2-(2-ACETYLAMINO-4-HYDROXY-6,8-DIOXA-BICYCLO[3.2.1]OCT-3-YLOXY)-PROPIONIC ACID | C11 H17 N O7 | 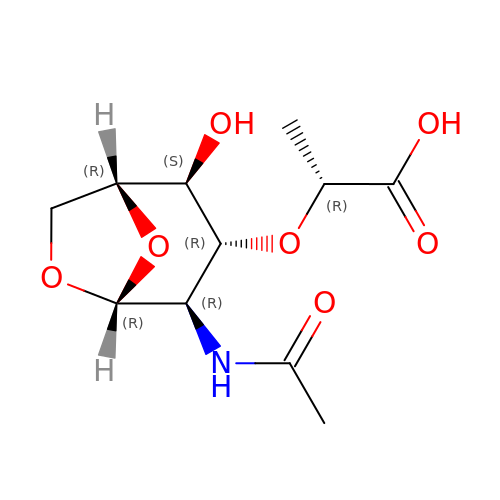ZFEGYUMHFZOYIY-YVNCZSHWSA-N>MEKKLEEVKQLLFRLELDIKETTDLLRNINKSIDQLDKYNYAMK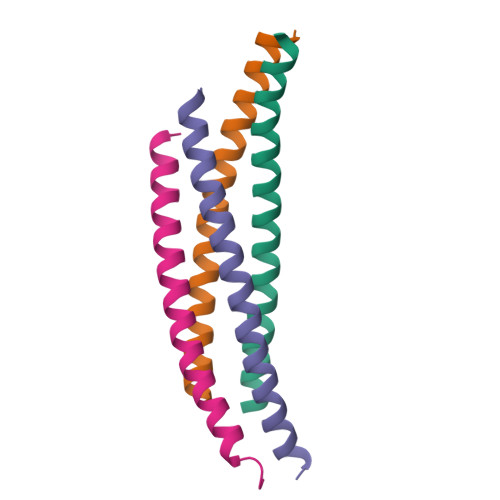IS[4x]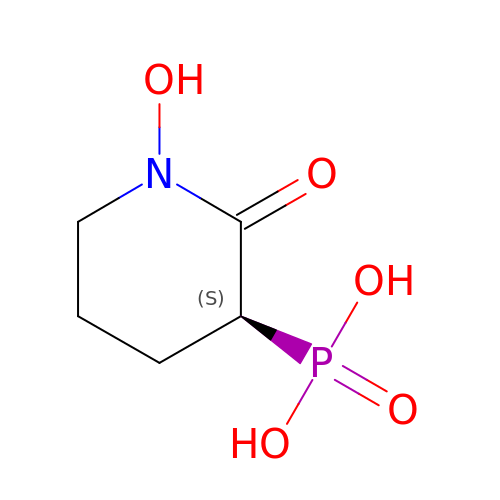[(3S)-1-hydroxy-2-oxopiperidin-3-yl]phosphonic acid | C5 H10 N O5 P | DVZQUMSQEGOYMX-BYPYZUCNSA-N> MLTAQTKNTQTLMPLTERVNVQADSARINQIIDGCWVAVGTNKPHAIQRDFTNLFDGKPSYRFELKTEDNTLEGYAKGETKGRAEFSYCYATSDDFKGLPADVYQKAQITKTVYHHGKGACPQGSSRDYEFSVYIPSSLDSNV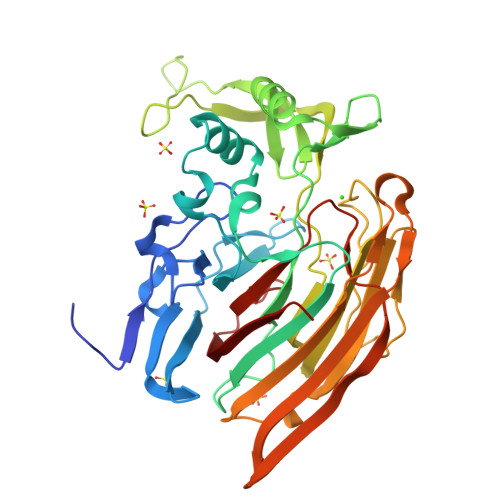STIFAQWHGMPDRTLVQTPQGEVKKLTVDEFVELEKTTFFKKNAGHEKVVRLDKQGNPMKDKNGKPVYKAGKLNGWLVEQGGYPPLAFGFSGGLFYIKANSDRKWLTDKDDRCNANPGKTPVMKPLTSEYKASTIAYKLPFADFPKDCWITFRVHIDWTVYGKEAETIVKPGMLDVRMDYQEQGKKVSKHIVNNEKILIGRNDEDGYYFKFGIYRVGDSTVPVCYNLAGYSERLE>MGLMNAFDSQTEDSSPAIGRNLRSRPLARKKLSEMVEEELEQMIRRREFGEGEQLPSERELMAFFNVGRPSVREALAALKRKGLVQINNGERARVSRPSADTIIGELSGMAKDFLSHPGGIAHFEQLRLFFESSLVRYAAEHATDEQIDLLAKALEINSQSLDNNAAFIRSDVDFHRVLAEIPGNPIFMAIHVALLDWLIAARPTVTDQALHEHNNVSYQQHIAIVDAIRRHDPDEADRALQSHLNSVSATWHAFGQTTNKKK[6x]

The Escherichia coli GntR-type transcriptional repressor, NanR, regulates sialic acid metabolism, but the mechanism is unclear. Analogous to other GntR members, the NanR monomer has a two-domain architecture, comprising an N-terminal winged helix–turn–helix DNA-binding domain (α1–α3, β1–β2, green) linked to an α-helical C-terminal effector-binding domain (α4–α10, tan). Here, we demonstrate that three NanR dimers bind a (GGTATA)3-repeat operator cooperatively and with high affinity. The effector, N-acetylneuraminate, binds NanR and attenuates the NanR-DNA interaction.

Initial two-dimensional classifications revealed two distinct populations: population 1 that had three NanR dimers bound to DNA, consistent with a NanR-dimer3/DNA hetero-complex; and population 2 that had a mixture of one or two NanR dimers bound to DNA. 3D reconstruction of the NanR-dimer3/DNA hetero-complex within population 1 revealed sufficient density for the (GGTATA)3-repeat operator and three NanR dimers, confirming the stoichiometry from our analytical ultracentrifugation experiments. We could unambiguously rigid body fit two NanR dimers, solved in our initial cryo-EM experiments, at either end of the DNA. However, density for the central NanR dimer had a lower signal-to-noise ratio and was consequently less resolved. Despite this, the middle NanR dimer could be confidently placed as densities corresponding to the flanking α2- and α2ʹ-helices of the N-terminal domain were observed when looking from the bottom of the DNA toward the dimer interface (inset). Analogous to the DNA-bound structure above, we observe that each NanR dimer sits in an asymmetric pose relative to the DNA, approximately a half turn away from each other, which aligns with the location of each GGTATA repeat within the operator sequence. Furthermore, we identified that the α3-helix made primary contact with the major groove, while the wing motif interacted with the minor groove of DNA across all three NanR dimers. Although the resolution of this dataset does not allow us to accurately locate the N-terminal extensions or confidently define their role in the assembly process, we note that they would be well placed to form protein–protein interactions with the adjacent NanR dimers to stabilize the complex. We believe the asymmetry in the DNA-binding pose is a prerequisite to accommodate further dimers of NanR, given the proximity we observe between each dimer within the NanR-dimer3/DNA hetero-complex, as they span the entire (GGTATA)3-repeat operator.> MGSSHHHHHHSSPISPIETVPVKLKPGMDGPKVKQWPLTEEKIKALVEICTEMEKEGKISKIGPENPYNTPVFAIKKKDSTKWRKLVDFRELNKRTQDFWEVQLGIPHPAGLKKKKSVTVLDVGDAYFSVPLDEDFRKYTAFTIPSINNETPGIRYQYNVLPQGWKGSPAIFQSSMTKILEPFRKQNPDIVIYQYMDDLYVGSDLE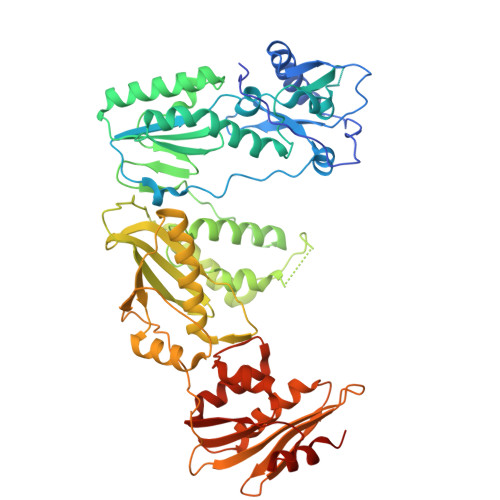IGQHRTKIEELRQHLLRWGLTTPDKKHQKEPPFLWMGYELHPDKWTVQPIVLPEKDSWTVNDICKLVGKLNWASQIYPGIKVRQLSKLLRGTKALTEVIPLTEEAELELAENREILKEPVHGVYYDPSKDLIAEIQKQGQGQWTYQIYQEPFKNLKTGKYARMRGAHTNDVKQLTEAVQKITTESIVIWGKTPKFKLPIQKETWETWWTEYWQATWIPEWEFVNTPPLVKLWYQLEKEPIVGAETFYVDGAANRETKLGKAGYVTNRGRQKVVTLTDTTNQKTELQAIYLALQDSGLEVNIVTDSQYALGIIQAQPDQSESELVNQIIEQLIKKEKVYLAWVPAHKGIGGNEQVDKLVSAGIRKVL> ASRSQAEDVRVEGSFPVTMLPGDGVGPELMHAVKEVFKAAAVPVEFQEHHLSEVQNMASEEKLEQVLSSMKENKVAIIGKIHTPMEYKGELASYDMRLRRKLDLFANVVHVKSLPGYMTRHNNLDLVIIREQTEGEYSSLEHESARGVIECLKIVTRAKSQRIAKFAFDYATKKGRGKVTAVHKANIMKLGDGLFLQCCEEVAELYPKIKFETMIIDNC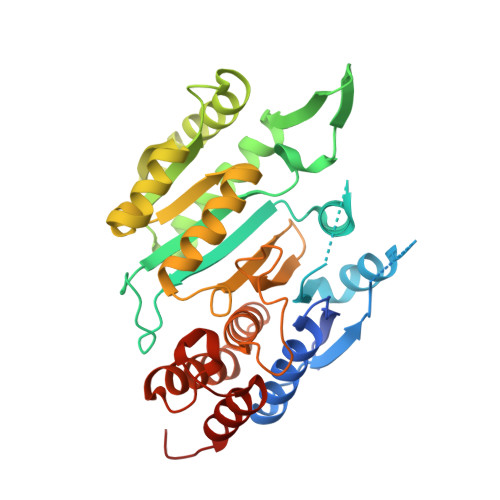CMQLVQNPYQFDVLVMPNLYGNIIDNLAAGLVGGAGVVPGESYSAEYAVFETGARHPFAQAVGRNIANPTAMLLSASNMLRHLNLEYHSSMIADAVKKVIKVGKVRTSDMGGYATCHDFTEEICRRVKDLDEN Members of the OSBP/ORP family vary in length: the short ORPs contain primarily a conserved OSBP-related domain (ORD) that can bind and transfer lipids such as sterols, PIPs or phosphatidylserine (PS), whereas the long ones often possess additional functional domains for ligand binding and/or membrane targeting. The OSBPL1A gene (homo sapiens) encodes two proteins: the long isoform ORP1L (residues 1–950) containing the ANK (ankyrin repeat) domain, the PH (Pleckstrin homology) domain, the FFAT (diphenylalanine in an acidic tract) motif and the ORD, and a short isoform ORP1S (residues 514–950) containing only the ORD. Here, while we cannot rule out its cholesterol sensor function, our structural, biochemical and cell biological data suggest that ORP1L is a bona fide cholesterol transporter. Here, our results suggest that ORP1 is a unique sensor of lysosomal PI-bisphosphates, and that PI(4,5)P2/PI(3,4)P2 allosterically regulates cholesterol transport by ORP1.

Nevertheless, we solved the PI(4,5)P2-bound structure using the direct mixture of ORP1-ORD and brain PI(4,5)P2. The binding mode of PI(4,5)P2 acyl chains is distinct from those observed in the PI4P-bound Osh structures. Nevertheless, the PI headgroup of PI(4,5)P2 nestles in a polar surface at the tunnel entrance, similar to that in the PI4P-bound Osh structures. The 4-phosphate group of PI(4,5)P2 interacts with the highly conserved His651 and His652 in the β2–β3 loop and Arg901 from helix α7, and the additional 5-phosphate group further interacts with His652 and the 4-phosphate group. The inositol ring and 1-phosphate group are engaged in contacts with several charged or polar side chains from the α4–β1 loop and α7 helix. Intriguingly, the inositol ring of PI(4,5)P2 is accommodated in ORP1-ORD with ~180° rotation compared with that of PI4P in Osh proteins; otherwise the 5-phosphate group would have caused a steric clash with helix α7. The rotatable property of the PI headgroup provides the possibility that ORP1-ORD can bind other PIPs such as PI(3,4)P2 that stimulates cholesterol transport as well. More significantly, the presence of such a charged, protruding group (5-phosphate) should interfere with the closure of the lid, which is likely to be very important for ORP1 functioning as a PI(4,5)P2- or PI(3,4)P2-dependent cholesterol transporter, similar to the case of another LTP32. Indeed, substitution of residues involved in PI headgroup recognition severely affected membrane targeting of ORP1-ORD. Last, cholesterol and PI(3,4)P2/PI(4,5)P2 (the PI headgroup) bind to the lipid-binding tunnel and the tunnel entrance of ORP1-ORD, respectively.

>[2x]MDALSNGIKKHRTSLPSPMFSRNDFSIWSILRKCIGMELSKITMPVIFNEPLSFLQRLTEYMEHTYLIHKASSLSDPVERMQCVAAFAVSAVASQWERTGKPFNPLLGETYELVRDDLGFRLISEQVSHHPPISAFHAEGLNNDFIFHGSIYPKLKFWGKSVEAEPKGTITLELLEHNEAYTWTNPTCCVHNIIVGKLWIEQYGNVEIINHKTGDKCVLNFKPCGLFGKELHKVEGYIQDKSKKKLCALYGKWTECLYSVDPATFDAYKKNDKKNTEEKKNSKQMSTSEELDEMPVPDSESVFIIPGSVLLWRIAPRPPNSAQMYNFTSFAMVLNEVDKDMESVIPKTDCRLRPDIRAMENGEIDQASEEKKRLEEKQRAARKNRSKSEEDWKTRWFHQGPNPYNGAQDWIYSGSYWDRNYFNLPDIYLEHHHHHH steviol-19-o-glucoside | C26 H40 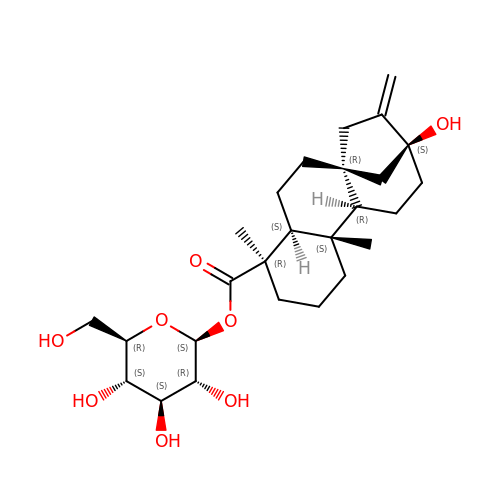O8 | OQPOFZJZPYRNFF-CULFPKEHSA-N>MAREVKLTKAGYERLMKQLEQERERLQEATKILQELMESSDDYDDSGLEAAKQEKARIEARIDSLEDVLSRAVILEEGTGEVIGLGSVVELEDPATGERLSVQVVSP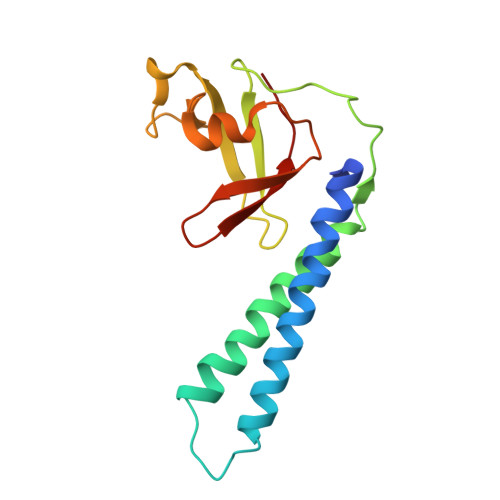AEASVLENPMKISDASPMGKALLGHRVGDVLSLDTPKGKKEFRVVAIHGR[3x]2-[[8-azanyl-7-fluoranyl-6-(8-methyl-2,3-dihydro-1~{H}-pyrido[2,3-b][1,4]oxazin-7-yl)isoquinolin-3-yl]amino]-6-propan-2-yl-5,8-dihydro-4~{H}-pyrazolo[1,5-d][1,4]diazepin-7-one 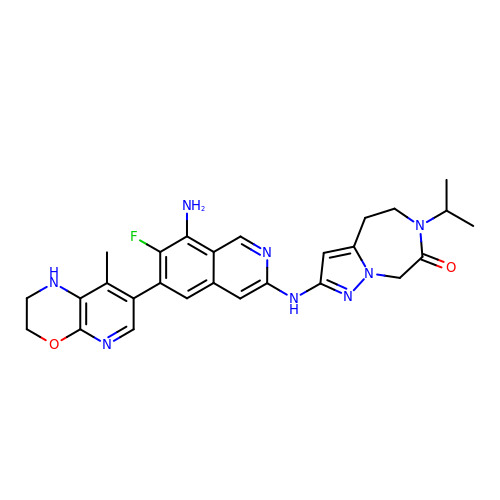| C27 H29 F N8 O2 | JOMBGXFENCGRHG-UHFFFAOYSA-N> MSDSVILRSIKKFGEENDGFESDKSYNNDKKSRLQDEKKGDGVRVGFFQLFRFSSSTDIWLMFVGSLCAFLHGIAQPGVLLIFGTMTDVFIDYDVELQELQIPGKACVNNTIVWTNSSLNQNMTNGTRCGLLNIESEMIKFASYYAGIAVAVLITGYIQICFWVIAAARQIQKMRKFYFRRIMRMEIGWFDCNSVGELNTRFSDDINKINDAIADQMALFIQRMTSTICGFLLGFFRGWKLTLVIISVSPLIGIGAATIGLSVSKFTDYELKAYAKAGVVADEVISSMRTVAAFGGEKREVERYEKNLVFAQRWGIRKGIVMGFFTGFVWCLIFLCYALAFWYGSTLVLDEGEYTPGTLVQIFLSVIVGALNLGNASPCLEAFATGRAAATSIFETIDRKPIIDCMSEDGYKLDRIKGEIEFHNVTFHYPSRPEVKILNDLNMVIKPGEMTALVGPSGAGKSTALQLIQRFYDPCEGMVTVDGHDIRSLNIQWLRDQIGIVEQEPVLFSTTIAENIRYGREDATMEDIVQAAKEANAYNFIMDLPQQFDTLVGEGGGQMSGGQKQRVAIARALIRNPKILLLDMATSALDNESEAMVQEVLSKIQHGHTIISVAHRLSTVRAADTIIGFEHGTAVERGTHEELLERKGVYFTLVTLQSQGNQALNEEDIKDATEDDMLARTFSRGSYQDSLRASIRQRSKSQLSYLVHEPPLAVVDHKSTYEEDRKDKDIPVQEEVEPAPVRRILKFSAPEWPYMLVGSVGAAVNGTVTPLYAFLFSQILGTFSIPDKEEQRSQINGVCLLFVAMGCVSLFTQFLQGYAFAKSGELLTKRLRKFGFRAMLGQDIAWFDDLRNSPGALTTRLATDASQVQGAAGSQIGMIVNSFTNVTVAMIIAFSFSWKLSLVILCFFPFLALSGATQTRMLTGFASRDKQALEMVGQITNEALSNIR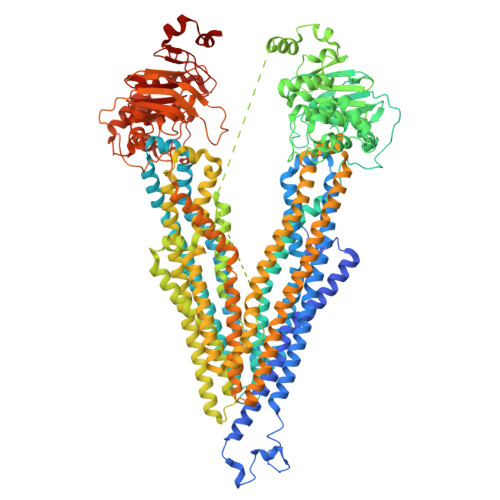TVAGIGKERRFIEALETELEKPFKTAIQKANIYGFCFAFAQCIMFIANSASYRYGGYLISNEGLHFSYVFRVISAVVLSATALGRAFSYTPSYAKAKISAARFFQLLDRQPPISVYNTAGEKWDNFQGKIDFVDCKFTYPSRPDSQVLNGLSVSISPGQTLAFVGSSGCGKSTSIQLLERFYDPDQGKVMIDGHDSKKVNVQFLRSNIGIVSQEPVLFACSIMDNIKYGDNTKEIPMERVIAAAKQAQLHDFVMSLPEKYETNVGSQGSQLSRGEKQRIAIARAIVRDPKILLLDEATSALDTESEKTVQVALDKAREGRTCIVIAHRLSTIQNADIIAVMAQGVVIEKGTHEELMAQKGAYYKLVTTGSPIS> MTSLNDIVNKLSSSKIKTRSDALQNLRSYIIYSRNGNSLNQEDALIIEKAIKRAFELEWQISANHGKRQISKASQEQKLQDISYLLRTCVESYILLFREPHILALLDIILRHTFTANGSICEVVCLNFSKALRLLLSHSPHLHHLRFSDWQSLVSYCCQAIEKLSIAEETYVSDSEEEPISQKNYQEISIWKSHDVIRVKQEVVELIYVMRSLVQWYAAPINFVSEQLLKFFEFFFYAYTEETDAHLPALQCLFQLCAYAIPNCNDYSASVVLLVFKILINSDKWKRLDLRLQLIQCLAISYPLWSNSETWDPHRSIRSFNLDLLNSSFFSLKNFLNFFGKRSSLSLANFRFHTVEPKNNIAKLYDPRLHLFFSLRHNSFFESYFIYFFLAKLILLKKTVLSLASTEQANKKQKTCSQIEELLLQAELANISASSFSLQLMVIITAISDNLTNDDLLSIQKMSLNFTEKKNELQSWSFFILFNICYNKAYSSMLTTSCKKEILAAASRGLLNSVTSPVCYQILTYFNMYRPLCFASIFPFIKQQFILFNDYSPMLSYEAIDYWKSLYILLNENLFVGQSSFKSVFLKWLKWHLYHLFSKEGELPFFSFTDSSIIIFDLLMMIFYRPLSLSYITTEIRSPFERNLFHLKEAWSPVTLRFPYTTDEICKQSTEGCYPFNSNHTIDCDSLQNVIKMLESSIDEISSASYDKDELDKETPSFEAVMIFSQISFLCGFLNCFIQKKGIHNVTPNNLVIFKNLFPEVLSFVKSNHSYDPIINCISTNLQFTISDEPKHLRYEIGSDLIRSTHFRDSNPLKTLVLYIMDMASKNVFIKPQEFDHDEYFSQEEEDIYRPENLIRNHQILGLMEGSLEQIRNTDLFILQKYIDYFSSHPHDSLINILHLYPIETFCFGMSAIGAYFLDVARTSEPIFYKCLEILAQKILMNYDYERDEVYLMIFIKIFQKCVHSKLQFTDATLKLIVKITKFIEKVFIETKFSSLSGRQTFLKFIFQLSPTSHVYSKFDYQKLISLTLKDSDVCVIYNFVDDLVIFLKKCDKTLIEGFVLPILSIKIEKSLYKGFCYLYLTLKVFLSISSNRSALLYQLLKLANSYETSTIFEPLLRKLHIQSANIKQLFRIYRLEIFWSFVSKDLSNTTNDFLEFPYKPIYFSLSDFLKENSDEIILVLILTKNITLAKLITSRMSVDFSEKYTQLIPVITTYTHLSEVENKKYSLRFNSIDEALDVELLNRSKAFLFCLEMLKEVKELGSTFKSISSTSFKVYSQLTIFANRVSFNNSTAIPFFSTKSVLWYCNRLFQELEGFSSIPSVIDLVLRRLAIQLHFATDEELQVTISFRLCAFLCFSDPFITSNYLVMIVLRIARQLLSIPCTQSLGLGIARFHLKKFKPTDFDYFFQLAEFCMDFLGFCYNTIGTKMEAIQDFYTWFDGYVTALLNFEYEGYGFLRCQINFVRSVMTTKNEWIEVSNKLFERGHFLKRIAMNNYLCLYFWQVLDACPRNVLHSLSLEIWKCYKAYDITEFPDSLKLFFSDIMGWNFFKSPEIADLNHYIPKTDPRLCDTKTYEESKLIIWKLICQKACSLLFKYDILLDSFIEDCIRMFFENGNHQELRKFLNFPKDSIIYDSDFKTLVSEEGSFQWVKLQPTNFDSLSNWTKEETLKLLNMMGKSSTTHSLKLLSTYMVGFSTSIIQYIIHLILLEFDFNGNNKKQKEYVTQLILSGLLNKNTNSIRKTCMNILLYLRRQLGHHALNPFEANYWVPINYSVAASTAYDCHLYEQSLLFLTIHNTKTDELDITLLSDILSQLPCPDAYYGIKRETSFKNILLKAVHEKRSPLAISYLDAANMYRSNEDEGTKMMFSNTLNNAGFFSLNEFYIDSLKANDAIDECSNEVYASAWRMQKWDIPPLSLDNKTTKDCLVFEVLHAVHNYAIYGNYLHLEEYINKKLLLINPNEEPDSLLFYALAYDLKFLIRCNQSQFNCDILQLLKENKQMSSQLHECFQLLLEIRNVLLSLLQSHKQLDLSDDLASFRKYYILELLKISESFLIVDNLQNAFSVAMLSDALYRKFDLADENLKHDIDFLSSKILWQRDEKIDAIGMLSESLSKTNSSIFPSISYAYLGNWLYTTKSEKTELVSKNYFEKSLSHMSHLNAKEKAKIYCMFAQFCDNNYSSPDLTEDFKRMEKLYFEKKNDIQQLERSIVNASNMKEEKMLKNHHSREMSSFIIDEREYLRMSTFRSKMLTQSITHYLKCLSESDENDVLISRCCTMWLSNSHLDELNNSLQHYLQNLPCKKFIPVFYQLAARLMNENSKFQQSLTSICYNVGRNHPYHSLHVLFSLVSNVPEIENLDAGSRYRAVKKILDLLKVNQGLSNLVTKLLCSFENYVSLAEWNPRSKVDSTSFSRFPGYKWFLKDAANYGLPPITMNVKVNDTGDYSNIPTVSSFDDTIHFASGINAPKVITCLGSNGHTYKQLVKGGNDDLRQDAVMEQVFEQVNGFLRSYRKTSQRNLSMRTYKVIPLALKTGVIEWVQDTIPLGEYLDSAHKVYHPKEWSLSTCRKLIAEKQMEDLETRLKVYDLVCRHYRPVFRHFFLESYADPVQWFTTQTNYARSTAVASVLGHVLGLGDRHGQNILIDKTSGEVIHIDLGIAFEQGKKLPVPECVPFRLTRDVVDGMGITGVEGVFRRCMEFTLETLRREEDSLLSVLEVLRYDPLFSWLISPLRRMKKQKMQLENFNQPESGNITTDASRDPKIQRNNVSGESEAERAILKVRQKLSSTLSVEASVGELIRIAQDPSYLALMFCGWSAFQ

The ataxia–telangiectasia mutated (ATM), an apical kinase that orchestrates the multifaceted DNA damage response, is the master regulator of genome stability, and is a critical therapeutic target in cancer. ATM/Tel1 kinase functions as an obligate homodimer with a highly dynamic N-terminal helical solenoid domain responsible for ligand binding and a conserved C-terminal FAT/kinase/FATC domain6. However, the activation mechanism of ATM/Tel1 in response to DNA damage remains largely unknown.

Previous cryo-EM structure of the ATM/Tel1 from Schizosaccharomyces pombe in the basal state has illustrated a dimer interface and the consecutive helical solenoids inhibiting the kinase activation. We show that ATM/Tel1 in the basal state adopts a symmetric dimer configuration with the kinase N-lobe suspended, keeping the N- and C-lobes misaligned, and the PRD fully ordered, blocking the substrate access to the active site. In its basal state, the PRD features fully ordered kα9b, kα9c, and the linker loop, which collectively create a complete obstruction to substrate access to the active site. This structural arrangement likely accounts for the significantly lower affinity of the CHK2 peptide to the basal-state ATM/Tel1. Upon activation, the Spiral shifts upward towards the FAT-Pincer, and the FAT harbors a coordinated conformational change, with the height reduced from 200 Å in the basal state to 164 Å. Two of the conformations, Structure 1 and Structure 3, which are closer to the basal and active states, respectively, do not bind to the substrate peptide. These structures were resolved at nominal global resolutions of 3.6 Å and 4.0 Å, respectively.> VGSLNCIVAVSQNMGIGKNGDYPWPPLRNEFRYFQRMTTTSSVEGKQNLVIMGKKTWFSIPEKNRPLKGRINLVLSRELKEPPQGAHFLSRSLDDALKLTEQPELANKVDMVWIVGGSSVYKEAMNHPGHLKLFVTRIMQDFESDTFFPEIDLEKYKLL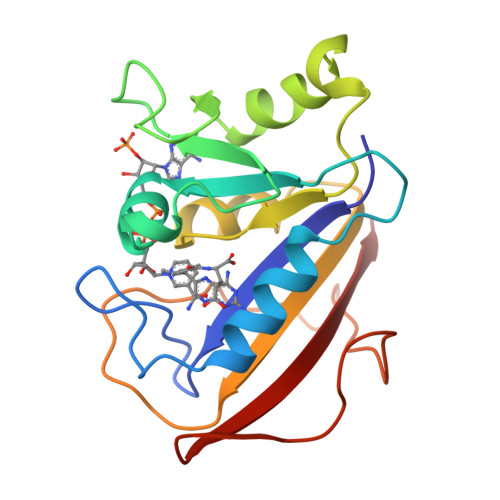PEYPGVLSDVQEEKGIKYKFEVYEKND4-{3-[2-amino-5-(2-methoxyethoxy)pyrimidin-4-yl]-1H-indol-5-yl}-2-methylbut-3-yn-2-ol 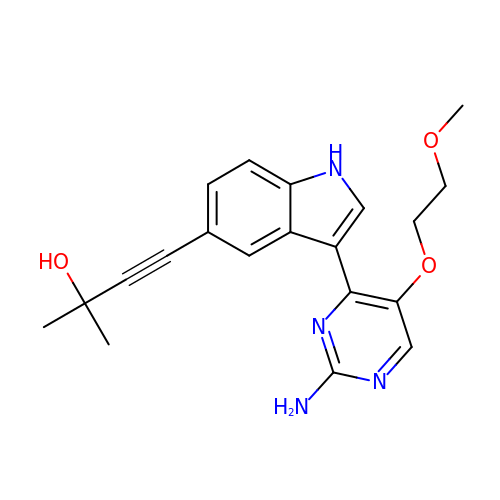| C20 H22 N4 O3 | ZZIZLABGKZWVAW-UHFFFAOYSA-N>[2x]GPLGSDEGVVKEIPITHHVKEGYEKADPAQFE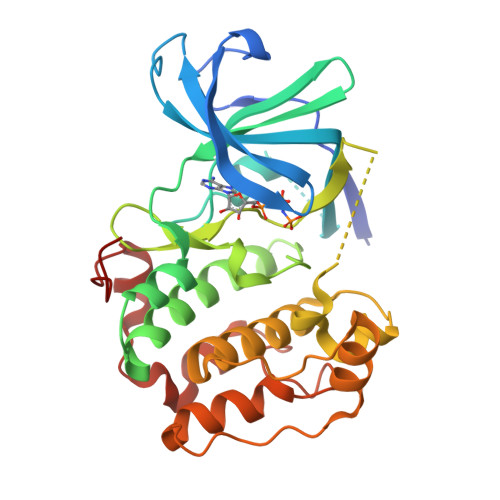LLKVLGQGSFGKVFLVRKKTGPDAGQLYAMKVLKKASLKVRDRVRTKMERDILVEVNHPFIVKLHYAFQTEGKLYLILDFLRGGDVFTRLSKEVLFTEEDVKFYLAELALALDHLHQLGIVYRDLKPENILLDEIGHIKLTDFGLSKESVDQEKKAYEFCGTVEYMAPEVVNRRGHSQSADWWSYGVLMFEMLTGTLPFQGKDRNETMNMILKAKLGMPQFLSAEAQSLLRMLFKRNPANRLGSEGVEEIKRHLFFANIDWDKLYKREVQPPFKP>AACAVDAGSVDQTVQLGQVRTASLAQEGATSSAVGFNIQLNDCDTNVASKAAVAFLGTAIDAGHTNVLALQSSAAGSATNVGVQILDRTGAALTLDGATFSSETTLNNGTNTIPFQARYFATGAATPGAANADATFKV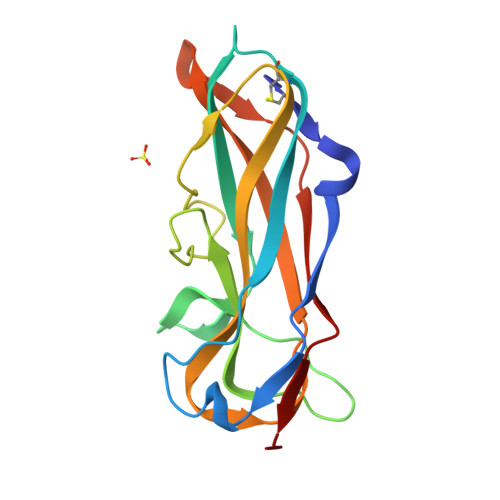QYQGGGGGGANVVEGKFHVTGGNVTTAA[8x]> MSKLTQVFKQTKLCIGYLTAGDGGTSYTIEAAKALIQGGVDILELGFPFSDPVADNPEIQVSHDRALAENLTSETLLEIVEGIRAFNQEVPLILYSYYNPLLQRDLDYLRRLKDAGINGVCVIDLPAPLSHGEKSPFFEDLLAVGLDPILLISAGTTPERMSLIQEYARGFLYYIPCQATRDSEVGIKEEFRKVREH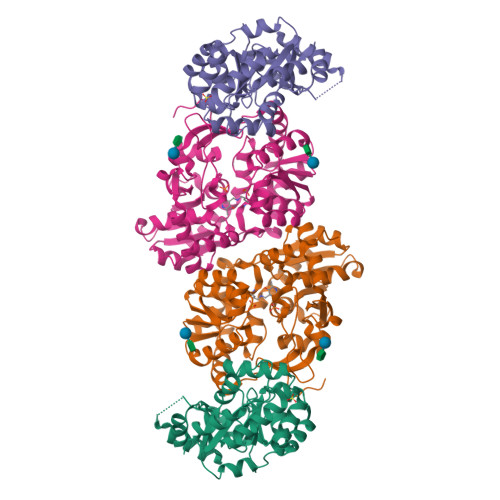FDLPIVDRRDICDKKEAAHVLNYSDGFIVKTAFVHQTTMDSSVETLTALAQTVIPG;> MFKHKHPFGGAFLPEELLAPIQNLKAEWEILKTQQSFLSELDCILKNYAGRQTPLTEVKNFARAIDGPRVFLKREDLLHTGAHKLNNALGQCLLAKYLGKTRVVAETGAGQHGVATATACAYLGLDCVVYMGAKDVERQKPNVEKMRFLGAEVVSVTKGSCGLKDAVNQALQDWATTHSFTHYCLGSALGPLPYPDIVRFFQSVISAEVKEQIHAVAGRDPDILIACIGGGSNAIGFFHHFIPNPKVQLIGVEGGGLGISSGKHAARFATGRPGVFHGFYSYLLQDDDGQVLQTHSISAGLDYPSVGPDHAEMHESGRAFYTLATDEEALRAFFLLTRNEGIIPALESSHALAHLVSIAPSLPKEQIVIVNLSGRGDKDLPQIIRRNRGIYE> ANPLYQKHIISINDLSRDDLNLVLATAAKLKANPQPELLKHKVIASCFFAASTRTRLSFETSMHRLGASVVGFSDSANTSLGKKGETLADTISVISTYVDAIVMRHPQEGAAR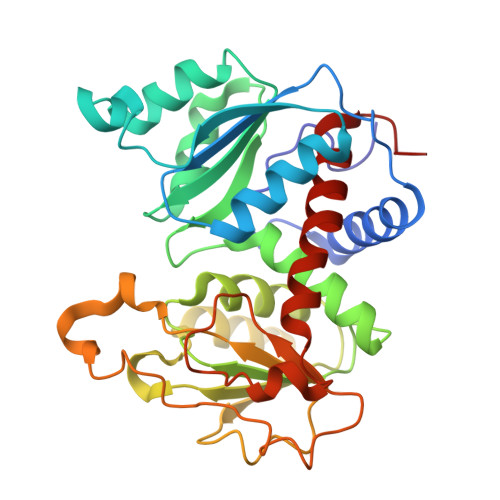LATEFSGNVPVLNAGDGSNQHPTQTLLDLFTIQETQGRLDNLHVAMVGDLKYGRTVHSLTQALAKFDGNRFYFIAPDALAMPQYILDMLDEKGIAWSLHSSIEEVMAEVDILYMTRVQKERLDPSEYANVKAQFVLRASDLHNAKANMKVLHPLPRVDEIATDVDKTPHAWYFQQAGNGIFARQALLALVLNRDLVL> TYMNNTEAICDAKGFAPFSKDNGIRIGSRGHIFVIREPFVSCSPIECRTFFLTQGSLLNDKHSNGTVKDRSPFRTLMSVEVGQSPNVYQARFEAVAWSATACHDGKKWMTVGVTGPDSKAVAVIHYGGVPTDVVNSWAGDILRTQESSCTCIQGDCYWVMTDGPANRQAQYRIYKANQGRIIGQTDISFNGGHIEECSCYPNDGKVECVCRDNWTGTNRPVLVISPDLSYRVGYLCAGIPSDTPRGEDTQFTGSCTSPMGNQGYGVKGFGFRQGTDVWMGRT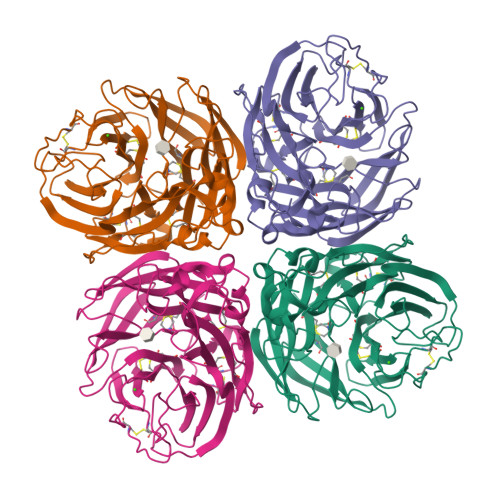ISRTSRSGFEILRIKNGWTQTSKEQIRKQVVVDNLNWSGYSGSFTLPVELSGKDCLVPCFWVEMIRGKPEEKTIWTSSSSIVMCGVDYEVADWSWHDGAILPFDIDKM>[2x]SNSITENTSWNKEFSAEAVNGVFVLCKSSSKSCATNDLARASKEYLPASTFKIPNAIIGLETGVIKNEHQVFKWDGKPRAMKQWERDLTLRGAIQVSAVPVFQQIAREVGEVRMQKYLKKFSYGNQNISGGIDKFWLEDQLRISAVNQVEFLESLYLNKLSASKENQLIVKEALVTEAAPEYLVHSKTGFSGVGTESNPGVAWWVGWVEKETEVYFFAFNMDIDNESKLPLRKSIPTKIMESEGIIGG

OXA-10 (PSE-2) is a class D β-lactamase that was originally described in the late 1970s and confers resistance to cefotaxime and ceftriaxone but not to ceftazidime. Natural and laboratory-selected variants of OXA-10 have been identified, many of which differ in the spectrum of β-lactams that they hydrolyze. Class D β-lactamases share the same general structure with conserved motifs, including an active-site serine 67, a carbamylated lysine (K70), and a stabilizing and invariant tryptophan residue (W154) within the Ω-loop. We were able to determine apo structures for both enzymes but not in complex with ceftazidime. Both protein structures contained two chains in the asymmetric unit, corresponding to a dimer, as previously described for OXA-10 (14, 24).

One such variant, OXA-14, contains a single amino acid change (glycine to aspartic acid at position 157, G157D) from the OXA-10 parent. The OXA-14 variant has been implicated in clinically significant resistance to ceftazidime. OXA-14 crystallized as a heterodimer in which, much like OXA-10, only one of the two K70 residues was carbamylated. In chain A of OXA-14, the Ω-loop was closer to the active site, and the indole group from tryptophan 154 (W154) interacted with the carbamylated lysine 70 (K70) (3.2 Å), as was described in OXA-10 (14). The interaction between W154 and K70 is critical for both the activity and the stability of OXA-10 (25). In chain B of OXA-14, K70 was decarbamylated, causing an open confirmation, consistent with what was observed for the heterodimeric structure of OXA-10 (14). The Ω-loop conformation was maintained, and the hydrogen bond between the indole group of W154 and K70 was present. We observed an increase in nitrocefin hydrolysis for OXA-14 as the pH value increased, suggesting that K70 was more stably carbamylated at a higher pH. Overall, OXA-14 hydrolyzed most of the tested β-lactams more efficiently than did OXA-935, specifically penicillin-G, cefepime, cephalothin, and cefotaxime. Compared to strains expressing the pPSV37 vector control, the expression of OXA-14 resulted in a 16-fold increase in the ceftazidime MIC and an 8-fold increase in the ceftazidime-avibactam MIC in PAO1 and a 16-fold increase in the MICs of both antibiotics in PA14, consistent with previous reports.>[2x]GLTPEQIIAVDGAHLWHPYSSIGREAVSPVVAVAAHGAWLTLIRDGQPIEVLDAMSSWWTAIHGHGHPALDQALTTQLRVMNHVMFGGLTHEPAARLAKLLVDITPAGLDTVFFSDSGSVSVEVAAKMALQYWRGRGLPGKRRLMTWRGGYHGDTFLAMSICDPHGGMHSLWTDVLAAQVFAPQV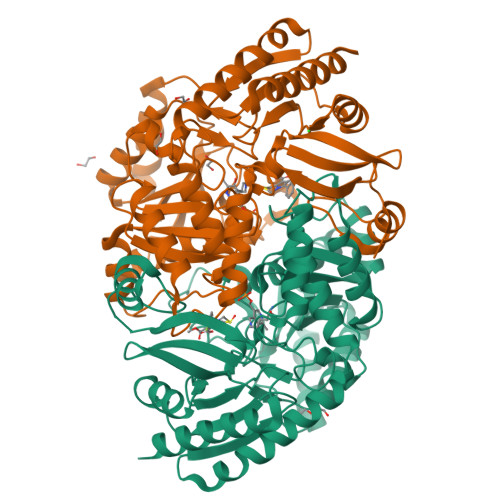PRDYDPAYSAAFEAQLAQHAGELAAVVVEPVVQGAGGMRFHDPRYLHDLRDICRRYEVLLIFDEIATGFGRTGALFAADHAGVSPDIMCVGKALTGGYLSLAATLCTADVAHTISAGAAGALMHGPTFMANPLACAVSVASVELLLGQDWRTRITELAAGLTAGLDTARALPAVTDVRVCGAIGVIECDRPVDLAVATPAALDRGVWLRPFRNLVYAMPPYICTPAEITQITSAMVEVARLVGS The large (L) protein of LASV is a multi-domain molecular machine that binds the conserved 3′ and 5′ ends (the ‘promoter’) of each of the two viral RNA (vRNA) genome segments (denoted L and S) and plays a central role in the viral life cycle, which is entirely cytoplasmic. The L protein contains an RNA-dependent RNA polymerase (RdRp) activity and catalyses both viral transcription and genome replication. Transcription is initiated using a capped primer derived from host mRNA by a yet to be elucidated ‘cap-snatching’ mechanism involving the intrinsic endonuclease (EN) of the L protein and possibly its cap-binding domain (CBD).

Two further structures were obtained from a sample in which the L protein was incubated with a truncated promoter (5′ nts 10–19, 3′ nts 1–19), which lacks nucleotides 0–9 of the 5′ end. One 3D class from this sample, obtained by focussed refinement on the promoter-bound region, (DISTAL-PROMOTER, 3.89 Å resolution), closely resembles the full promoter (PRE-INITIATION) structure, but additionally reveals a new position of the EN, without inhibitory peptide bound. In the MID-LINK and DISTAL-PROMOTER structures, the EN has flipped by ~160° around a hinge between G195-G199. The EN active site faces away from the rest of the polymerase and is exposed to the solvent, free of the inhibitory peptide. Instead, inhibitory peptide residues 1087–1099, as well as PB2-like segments 1759–1770 (lid), 1852–1860 and 1894–1896 (mid), 2077–2081 and 2089–2091 (link) pack against the back of the EN, stabilising it in its new location. Similarly, the α-bundle of MACV apo-L (with its different topology) superposes with the pendant domain in LASV L, showing that these flexible and linked domains must rearrange from the apo-state observed in MACV L. Finally, the position of the pendant domain in the LASV PRE-INITIATION structure is incompatible, due to significant steric overlap, with the location of the inhibited EN in the APO-ENDO or 3END-ENDO structures. This important observation provides a plausible rationale for full promoter binding (as opposed to just the 3′ end binding in the secondary site) inducing a flip of the EN to the alternative uninhibited location observed in the MID-LINK and DISTAL-PROMOTER structures (see above).

> MEDDMACVKDLVSKYLADNERLSRQKLAFLVQTEPRMLLMEGLKLLSLCIEIDSCNANGCEHNSEDKSVERILHDHGILTPSLCFVVPDGYKLTGNVLILLECFVRSSPANFEQKYIEDFKKLEQLKEDLKSVDINLIPLIDGRTSFYNEQIPDWVNDKLRDTLFSLLRYAQESNSLFEESEYSRLCESLSMTSGRLSGVESLNVLLDNRSSHYEEIIASCHQGINNKLTAHEVKLQIEEEYQVFRNRLRKGEITGQFLKVDKSRLLNDFNNLYVDEVTATKDNIEHLIYQFKRASPILRFLYANIGEGNGEERHHTIKECQMQYWRSFLNKVKSLRILNTRRKLLLIFDALILLASIHDQTRHKCSKGWLGSCFISVNDRLVSLESTKRDLEKWVGRRQQSERSNTIQPPDKNQILISMFQKTILKATAALKDVGISVEHYKINMEVICPDSYDLILNFDVSGVVPTISYQRTEDEKFPFIMGGVELLESTDLERLSSLSLALVNSMKTSSTVKLRQNEFGPARYQVVRCKEAYCQEFLLSGAEFQLIYQKTGECSKCYAINDNRVGEICSFYADPKRYFPAIFSAEVLQTTVSTMISWVKDCSELEEQLCNINSLTKMILVLILAHPSKRSQKLLQNLRYFIMAYVSDYHHKDLIDKLREELITDVEFLLYRLVRALVNLILSEDVKSMMTNRFKFILNISYMCHFITKETPDRLTDQIKCFEKFLEPKLEFGHVSINPADVATEEELDDMVYNAKKFLSKEGCTSIKGPDYKKPGVSKRFLSLLTSSFNNGSLFKESEVKREIKDPLVTSGCATALDLASNKSVVVNKYTDGSRVLNYDFNKLTALAVSQLTEVFSRKGKHLLNKQDYDYKVQQAMSNLVLGPRQNKVGADEADLDEILLDGGASVYFDQLKETVERIIDQYREPVKPGSNPNGGDQPSVNDLDEVVPNKFYIRLIKGELSNHMVEDFDYDVLPGNFYEEFCDAVYKNNKLKERYFYCGQMSQCPIGELTKAVATRTYFDQEYFQCFKSILLIMNANTLMGRYTHYKSRNLNFKFDMGRLSDDVRISERESNSEALSKALSLTNCTTAMLKNLCFYSQESPQSYSSTGPDTGRLKFSLSYKEQVGGNRELYIGDLRTKMFTRLIEDYFEALSLQLSGSCLNNEREFENAILSMKLNVSLAHVSYSMDHSKWGPMMCPFLFLATLQNLIFLSKDLQADIKGRDYLSTLLTWHMHKMVEIPFNVVSAMMKSFIKAQLGLKKKTTQSITEDFFYSNFQIGVVPSHVSSILDMGQGILHNTSDFYALISERFINYAISCICGGTIDAYTSSDDQISLFDQVLTELMQRDPEEFKTLIEFHYYMSDQLNKFVSPKSVIGRFVAEFKSRFYVWGDEVPLLTKFVAAALHNIKCKEPHQLAETIDTIIDQSVANGVPVHLCNLIQKRTLSLLQYARYPIDPFLLNCETDVRDWVDGNRSYRIMRQIERLIPDACGRIRSMLRKLYNKLKTGQLHEEFTTNYLSSEHLSSLSNLCELLGVEPPSESDLEFSWLNLAAHHPLRMVLRQKIIYSGAVNLDDEKVPTIVKTIQNKLSSTFTRGAQKLLSEAINKSAFQSSIASGFVGLCRTLGSKCVRGPNKESLYIKSIQSLISDIQGIEPLIDSHGVQYWRVPLNIRDGNEGVISYFRPLLWDYMCISLSTAIELGAWVLGEPKKVRVLEFFKHNPCDYFPLKPAASKLLEDRVGLNHIIHSLRRLYPSVFEKHILPFMSDLASTKMKWSPRIKFLDLCVALDVNCEALSLVSHIVKWKREEHYIVLSSELRLSHTRTHEPMVEERVVSTSDAVDNFMRQIYFESYVRSFVATTRTLGSFTWFPHKTSVPEGEGLQRLGPFSSFVEKAIHKGIERPMFKHDLMMGYAWIDFDIEPARFNHNQLIASGLVGPRFDSLEDFFDAVESLPPGSAKLSQTVRFRIKSQDASFKESFAIHLDYTGSINQQTKYLVHEVSAMYSGAVSPCVLSDCWRLVLSGPTFKGKSAWYVDTEIVNEFLTDTNQLGHVTPVEIVVDMEKLQFTEYDFVLVGPCVEPVPLVVHRSGLWECDKKLASFTPVVQDQDLEMFVKEVGDSSLDLLIGALSAMILDRLKLRMQWSEVDIVSMLKAAMPSNSVKVLNAVLEAVDDWVDFKGYALCYSKSRKKVMVHSSGGKLRLKGRTCEELVKEDEGIEDIE> ETGQVAASPSINVALKAAFPSPPYLVELLETAASDNTTIYYSLLDRIAKGHFAEATTDKALYEKFLEVLRDDGHMDPEALSAFKLALSLRTATPRVEAHYQYYTATVEPSLSGTQEGCDQWFLIDGEQYCSPTLDTSHGKVKGEDQLRTLPFDRKFGVGCRDVILYADITSKSFAPFHEVAMDLAKKGKASYRVRYRRSPSHSRESLSVNGYGVELVLKRTDYIVIDDRDTGAAAKPAEENDQKPLVGHETVLDDGEEIADIKPLEKSELAALGMKAASFVMQSEKPFEALLKLTQDFPKYSNSLGSQNVSAEFEAEHRGNREVFLPEGSNVLWLNGLHLIDRQIQPFGLVDLLTRERKLIKSVLDLGLTGQQAVDLLGHAEVAHAKSGDDEPRRFDWRDDIEEGQVIIWLNNLEKDKRYKS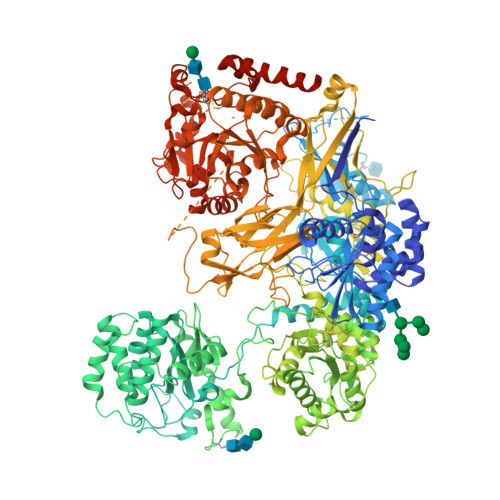FSPSIWVLIHHFGHGLPQIRRDVFNLVVPVDLTKADDVKIVVEGLLSFVKRLIPVRFGFVPLTPTGQAIDQAKVVYYLLENYGLAAATAYLEKSYEEQSTGQPNERIFNEVIKDKSLRPDGVELSFKDIFISEKHEKQIHLSKHWVERLRAGGDVPTVFFDGFPIPREDNWLRVMNHRLMQDLQALQQAGYFGMLNESMWLPGFFLEKALSRRNTLIFPEDKNELTVLNVNKIYIENHDLMSKVPVIEASKESTRDDWAALTVVADLDDIEGQELVYYALRFRKSNDGVRLDIVHNPKDCSRSPSVLAQRLKSREDKLLDFTRFLDLETALETGEFEPDVAYDASLANFLASSNMKAGDNFVILNGRVLGPITSADDFKKEDFEVFLQAERRTRILPVYKALEDLGLDDKVSGPLSAAKLTSVTALSTISDLPQGIFDNAPTVRTTLFKQWNSTYTSFEVGDASTATIFFVAVINPASEIGQRWVAVLKVLSELEGVHLRVFLNPTVMIEELPVKRFYRYVLSSSPSFDESGKVKALSARFTGVPRETLLVVGMDVPPAWLVTSKVAVDDLDNLRIKDIKAKRGTEHVEAIYELEHILIEGHSREIPGAHAPRGVQLVLETENNPHFADTIIMANLGYFQFKANPGVYNIRLKEGRSSEIFTLESVGAKGWGPIPGDDNTEVVLMDFQGTTLYPRLRRKPGMEEEDVLEPSTKSGEESGSGARNLVSRGIKFAEGLLGRGNKAAEATKSVSKTEHAEINIFSVASGHLYERMLNIMMASVMHHTNHTVKFWFIEQFLSPSFKDFIPHMAAEYGFKYEMVTYKWPHWLRQQKEKQREIWGYKILFLDVLFPLSLDKVIFVDADQIVRTDMYDLVEHPLDGAPYGFAPMCDSRVEMEGYRFWKTGYWANYLKGKPYHISALYVVDLQRFRELAAGDRLRQQYHALSADPNSLANLDQDLPNHMQFTIPIATLPQEWLWCETWCSDETLKDARTIDLCNNPMTKEPKLDRARRQVPEWTKYDEEIAELARRVREEKPKKKEEEKVQKNPKSRRLDGDEEEVKTVREGTKHHHHHH>EFMSTTDAPDLSAQIAAELPYLRRYARALTGSQSSGDAYALATLEAILDEPALFETGTTPRVALFTVFHTIWNSSGSPVSDGETGLARAAQRHLARLTPNTREALLLSTIEDFTPEEVATIMRSDVDEVRHLINRARSEMEDSVSGRVMIIEDEAIIALDLQTIVADMGHAITGVARTRDAAVALAGIEKPDLILADIQLADRSSGIDAVNEILRARGDIPVIFITAFPERLLTGERPEPAFLISKPYREDQVRSAISQAMFFASTEPLKA[3x]

The GSR is a gene expression program that enables bacteria to cope with a range of adverse conditions such as oxidative stress, heat shock, and UV exposure. This response works using a so-called “partner-switching” mechanism, whereby HK activity—and subsequent phosphorylation of a downstream PhyR regulator —controls the activity of a transcriptional inhibitor known as NepR. Stress activates an HWE/HisKA2 HK, phosphorylating the PhyR and promoting sequestration of NepR away from σEcfG, allowing transcription of stress-responsive genes to occur. Exploring downstream effects of RT-HK, we identified two homologs of PhyR in the genome, RT-PhyR and RT-PhyR′. In the structures of both RT-PhyR and RT-PhyR′, we observed a typical arrangement between the SL and REC domains.

RT-PhyR and RT-PhyR′ were solved as a crystallographic trimer and a tetramer, respectively. Aligning the two PhyR paralog structures shows a reasonably high degree of overall similarity (2.7 Å Cα RMSD), with a notable major shift in the position of the loop connecting the β3 strand (immediately following the phosphoacceptor aspartate) and subsequent α10 helix (α3 in standard REC nomenclature). The propensity for the unphosphorylated PhyR homologs to bind RT-NepR′ may be related to the density for the typically flexible α4 helix seen in the RT-PhyR structure. Alignment of the RT-PhyR SL domain with PhyR structures from other organisms reveals a shift in this region where its α4 helix is situated between the expected NepR-bound and unbound positions. However, we are wary of overinterpreting this particular detail, as intermolecular interactions between RT-PhyR molecules in the crystal involve the α4 helix, so this position may be artificially stabilized. At the short timepoint, we observed transfer only to RT-PhyR, suggesting that it is the cognate partner of RT-HK. Further, the intensity of the phosphorylated RT-PhyR bands were higher in the dark condition at both timepoints, indicating RT-HK’s reversed logic had been transferred downstream. For RT-PhyR, we saw many peaks shift into positions distinct from those seen when the protein was titrated with either substance alone, indicating a synergistic effect. In RT-PhyR, these two pathways from the unphosphorylated conformation evidently act synergistically to promote formation of the final phosphorylated RT-NepR′-bound complex, as previously proposed for Caulobacter crescentus.(2~{R})-1-[(2~{R})-1-(2-methoxyethoxy)propan-2-yl]oxypropan-2-amine | C9 H21 N O3 | 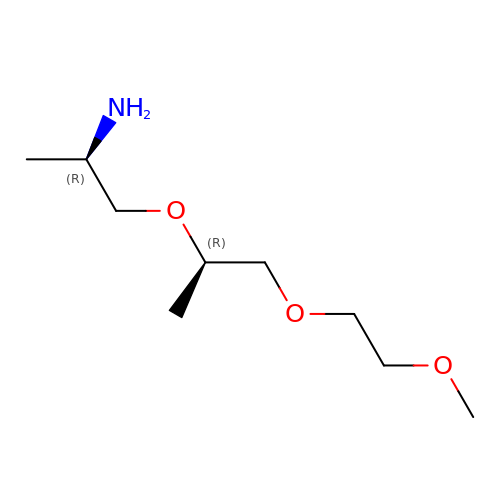JKCPHDAMWZLSSR-RKDXNWHRSA-N> ETGTPMMPPVGVQASILSHDTIRITWADNSLPKHQKITDSRYYTVRWKTNIPANTKYKNANATTLSYLVTGLKPNTLYEFSVMVTKGRRSSTWSMTAHGATFELVPTSPPKDVTVVSKEGKPRTIIVNWQPPSEANGKITGYIIYYSTDVNAEIHDWVIEPVVGNRLTHQIQELTLDTPYYFKIQARNSKGMGPMSEAVQFRTPKADSSDKMPNDQALGSAGKGSRLPDLGSDYKPPMSGSNSPHGSPTSPLDSNGTKHHHHHH;> QAKHKQRKRLKSSCKRHPLYVDFSDVGWNDWIVAPPGYHAFYCHGECPFPLADHLNSTNHAIVQTLVNSVNSKIPKACCVPTELSAISMLYLDENEKVVLKNYQDMVVEGCGCR;> ETGQPAQCRIQKCTTDFVSLTSHLNSAVDGFDSEFCKALRAYAGCTQRTSKACRGNLVYHSAVLGISDLM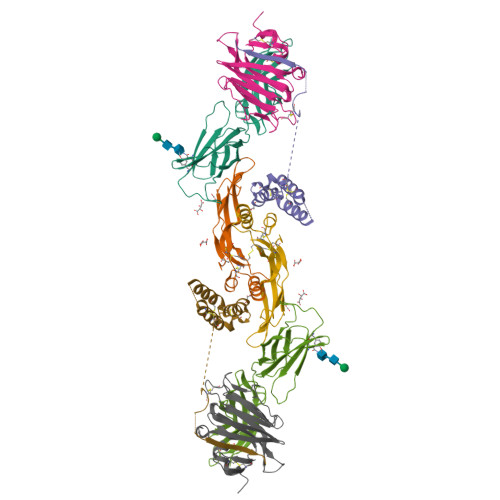SQRNCSKDGPTSSTNPEVTHDPCNYHSHAGAREHRRGDQNPPSYLFCGLFGD;> PHLRTFKDNFQTCKVEGAWPLIDNNYLSVQVTNVPVVPGSSATATNKITIIFKAHHGCTDQKVYQAVTDDLPAAFVDGTTSGGDSDAKSLRIVERESGHYVEMHARYIGTTVFVRQVGRYLTLAIRMPEDLAMSYEESQDLQLCVNGCPLSERIDDGQGQVSAILGHSLPRTSLVQAWPGYTLETANTQCHEKMPVKDIYFQSCVFDLLTTGDANFTAAAHSALEDVEALHPRKERWHIFPSGTKHHHHHH> G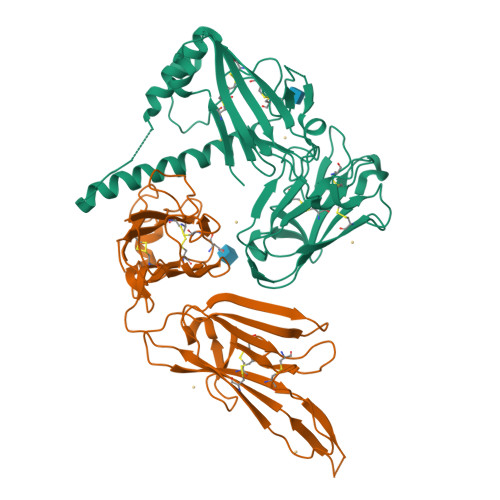ASKSHKCDFTKEKYLLSGEKEVSCEIDANPSDDITFICPNKIDSLCFHTVNISKNINQNKSTMSIQDLLYGSVVYGNTLFISPYVRTNTPFYCFCNLDTVTIQKFLKINRFLKDDDELSEADVMKHLKGGNVSEAQADEYLNKALNRFKKMKDLSKFFNDQADNTTKLNLPKSLNIPNDILNYDVYNSSNNRNDIVVKDEVTNKQIISKRGIMSVFVRSNNNVIKGCDFGNNNKNYFSHPISVAGKVNNKVCKIQGKPGELVGFKCAFEENGKVEPPNCFDQVLHKNKVTDLKTLIPGYASYTNKHSSKYPYYLKIPHFVNEQYTIQCKCKSNNSQNEYTFELDIQPGES;> GASNLTCDFNDVYKLEFHPNQQTSVTKLCNLTPNVLEKVTIKCGSDKLNYNLYPPTCFEEVYASRNMMHLKKIKEFVIGSSMFMRRSLTPNKINEVSFRIPPNMMPEKPIYCFCENKKTITINGSNGNPSSKKDIINRGIVEIIIPSLNEKVKGCDFTTSESTIFSKGYSINEISNKSSNNQQDIVCTVKAHANDLIGFKCPSNYSVEPHDCFVSAFNLSGKNENLENKLKLTNIIMDHYNNTFYSRLPSLISDNWKFFCVCSKDNEKKLVFTVEASISS>ATHEVHMLNKGESGAMVFEPAFVRAEPGDVINFVPTDKSHNVEAIKEILPEGVESFKSKINESYTLTVTEPGL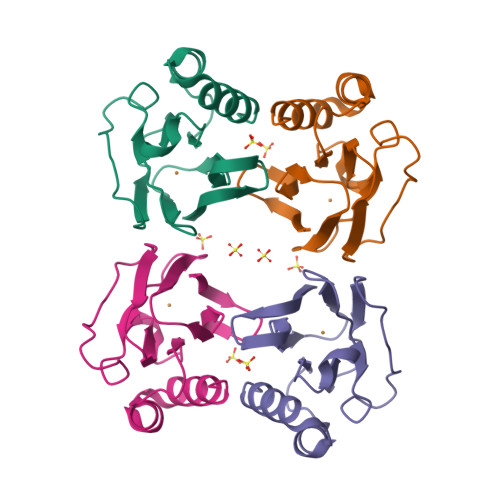YGVKCTPHFGMGMVGLVQVGDAPENLDAAKTAKMPKKARERMDAELAQVN[2x]>SVGTFSLPALPYAYDALEPSISAQIM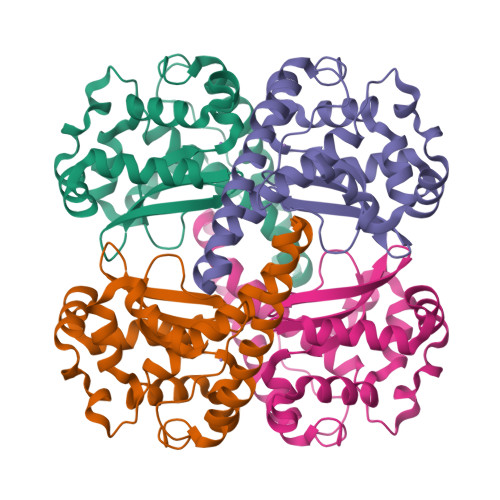ELHHSKHHQTYVTNLNNALKTYSTALAANDVPSQIALQAAIKFNGGGHINHSFFWENLCPASSPDADPASAPELTAEIAKTWGSLDKFKEAMGKALLGIQGSGWGWLVKEGSGLRIVTTKDQDPVVGGEVPVFGIDMWEHAYYLQYLNGKAAYVDNIWKVINWKTAEQRFKGDREDAFKILKASL[6x]>[2x]MKTIKMVADELNVTKQTVVNNAKNLNISFEKENGVNYIDDNDYLKIVEKITKKERTTQNKENKKSEITYENTEKNRYNNSDGF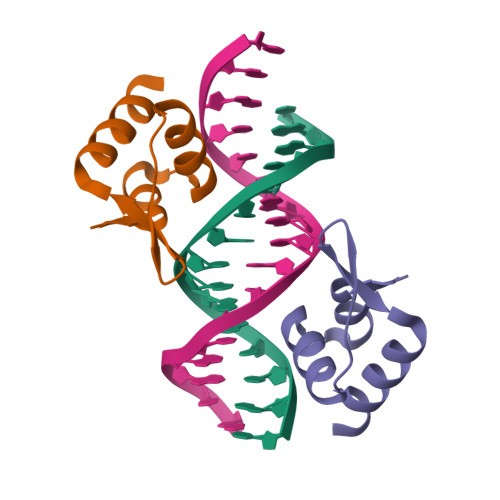ETLKTKVNELEKQVEIFETRAKNDEKYIENLTKQLDQQNSNVNTLNKLLENQQILALESNKKIQKLEHQLEEERQLSYSFDKSTNDR>[4x]AFRIPLTRFKSVRKQLAEEGIYIHEGPYPEPLVNLLDVVYYGPISIGTPPQDFQVIFDTGSANLWLPSSKCTTKYCLHHHRYDSSKSSTYEADGRNFTIVYGSGNVEGFISKDVCRIGSAKVSGQPLGEALVVG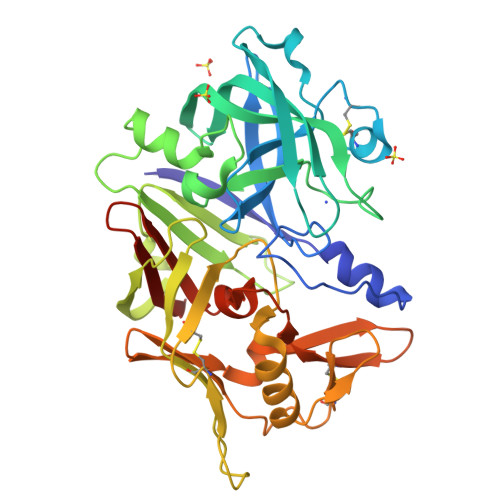GESLLEAPFDGILGLAYPSIAVDGVVPVFDNMMKQGLLGEQNVFSVYLNRDPSSKEGGEVLFGGIDHDHYKGSITYVPVTAKGYWQFHVDGVKSVSASKSAPELLCKDGCEAIANTGTSLITGPPEEVDSLNQYLGGTKTEGGQYLLDCDKLESLPNVTFTISGKEFSLRSKDYVLKVNQQGQTLCVSGFMGLEMPQPLWILGDVFLGPYYTIFDRDQDRVGFAEVAHHHHHH>MAKYFGTDGIRGEVANSTITVEFTQKLGNAVGSLINQKNYPKFVIVGQDTRSSGGFLKFALVSGLNAAGIDVLDLGVVPTPVVAFMTVKHRAAAGFVITASHNKFTDNGIKLFSSNGFKLDDALEEEVEDMIDGDFIYQPQFKFGSYKILANAIDEYIESIYSRFAKFVNYKGKVVVDCAHGAASHNFEALLDKFGINYVSIASNPDGLNINVGCGATCVSNIKKAVKEQKADLGISLDGDADRIIIVDENGQEIDGDGILNIL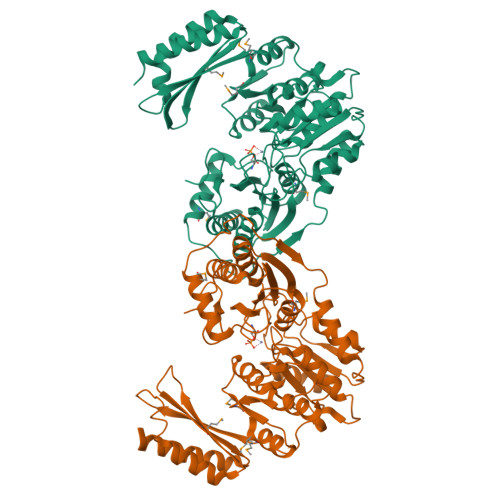AQYSDICGGTNGIVGTQMTNMSYENHYRANKIPFIRSKVGDRYVLEDLVKYGYKIGGESSGHVINLNFGTTGDGLFTAIQLLAIFSQADKPVSEFKLQGELMQQTLINVPLTKKVAREDLQKVASDVNDVEKRLGNRGRVLLRPSGTEPVLRVMVEADDKSLATNEAEYLVEKVKQKLV[2x]>GSHMTPDIILQRTGIDVRAVEQGDDAWHKLRLGVITASEVHNVIAKPRSGKKWPDMKMSYFHTLLAEVCTGVAPEVNAKALAWGKQYENDARTLFEFTSGVNVTESPIIYRDESMRTACSPDGLCSDGNGLELKCPFTSRDFMKFRLGGFEAIKSAYMAQVQYSMWVTRKNAWYFA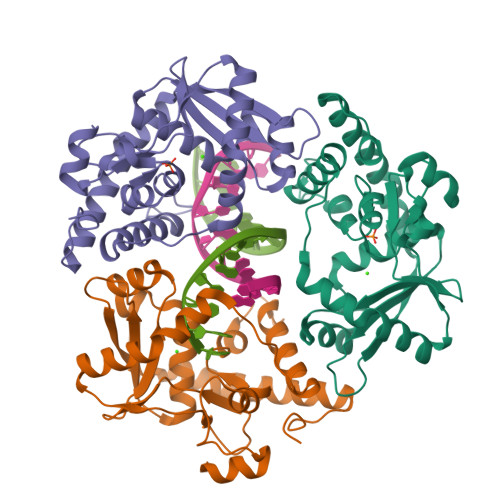NYDPRMKREGLHYVVIERDEKYMASFDEIVPEFIEKMDEALAEIGFVFGEQWR[3x]>[2x]GPYLQILEQPKQRGFRFRYVCEGPSHGGLPGASSEKNKKSYPQVKICNYVGPAKVIVQLVTNGKNIHLHAHSLVGKHCEDGVCTVTAGPKDMVVGFANLGILHVTKKKVFETLEARMTEACIRGYNPGLLVHSDLAYLQAEGGGDRQLTDREKEIIRQAAVQQTKEMDLSVVRLMFTAFLPDSTGSFTRRLEPVVSDAIYDSKAPNASNLKIVRMDRTAGCVT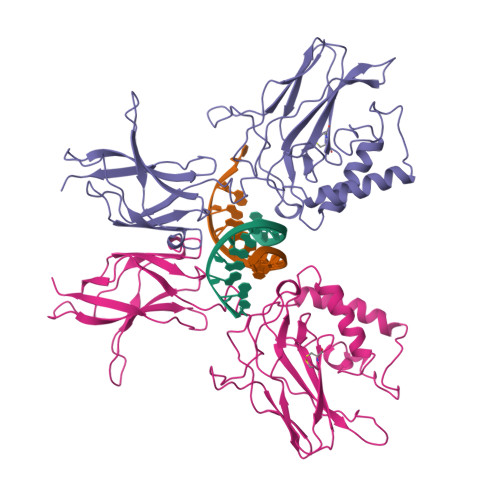GGEEIYLLCDKVQKDDIQIRFYEEEENGGVWEGFGDFSPTDVHRQFAIVFKTPKYKDVNITKPASVFVQLRRKSDLETSEPKPFLYYPEIKDKEEVQRKRQK>ETGKDTAFVEVVLFESSPNGDYTTYTTGLQGRFSRAGATISAEGEIVQMHPLGLCNNNDEEDLYEYGWVGVVKLEQPELDPSCLTVLGKAKRAVQRGATAVIFDVSENPDAIDQLNQVSEDPLKRPVVYVKGADAVKLMNIVNKQKVARARIQHRGTKHHHHHH[2x]

Rspo (R-spondin, also roof plate-specific spondin) proteins are evolutionarily conserved from fish to humans and have well-documented roles in a broad range of developmental and physiological processes resulting from enhancement of canonical and non-canonical Wnt signalling. ZNRF3/RNF43 specifically targets these Wnt receptors for ubiquitination and turnover, hence reducing Wnt signalling responses. Direct extracellular interaction with Rspo proteins inhibits ZNRF3/RNF43 activity. Here we report a molecular level analysis of the ZNRF3/RNF43 ectodomain structure and its interactions with Rspo proteins.

The ZNRF3ecto crystal structures revealed a distinctive variant of the protease-associated domain topology. Two β-sheets (comprising β2, β1, β7, β3 and β4, β5, β6 strands, respectively) splay apart, accommodating an α-helix (αC) at the open edge; two additional α-helices (αA and αB) pack against the β4, β5 and β6 face of this distorted β-sandwich. A disulphide bridge, conserved across species, links two structurally elaborate loops, β3–β4 and β4–αA. The crystal structures for apo xZNRF3ecto, zZNRF3ecto and mZNRF3ecto showed no major differences in the main chain conformation. Comparisons of ZNRF3ecto structures for proteins crystallized in several different crystal lattices, or for crystals containing multiple copies in the asymmetric unit, consistently highlighted an acidic region (N105-E114; residue numbering is for mouse sequences unless otherwise stated) within the β3–β4 loop, the short αC–β7 loop and the extended β1–β2 hairpin as flexible elements of the fold. Our crystallographic data provided independent structures for multiple copies of the ZNRF3 ectodomain in eight different crystal forms. All but two of these crystal structures reveal an extensive interface (average interface area 992±109 Å2) formed between two ZNRF3ecto polypeptide chains. This dimer is conserved, and pairwise structural superpositions yielded r.m.s.d. values of <1.3 Å (for 275 equivalent Cα pairs). The interaction is twofold symmetric; strands β3 and β7 of the ‘subunits’ abut face-to-face at the core of the dimer. The β1–β2 hairpin forms a second interface by reaching out to embrace helix αA and the β3–β4 loop in the opposing subunit.> MRME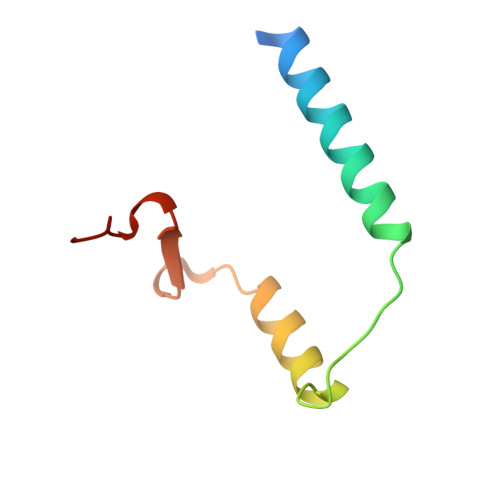KVGDVLKELERLKVEIQRLEAMLMPEERDEDITEEEIAELLELARDEDPENWIDAEELPEPED> MKSRLKQQIFAISLLACTAISPANALQTHLLREQFQNPSDEAKPWTFWYWMFGAVSKEGITADLEAMKRAGLGGTYLMPIKGIKEGPQYNGKAQQLTPEWWEMVRFSMEEADRLGLKLGMHICDGFALAGGPWMTPKESMQKIVWSDTIVDGGKIKGLHLPQPEAYEGFYEDISLFALPVKEEAADVMPAQITCANIATGNHIDIKKTVNMDDAGVIRSSYPCYIQYEYEQPFTCRNIEIILSGNNYQAHRLKVMASDDGVNYRLVKQLVPARQGWQNTDENSTHAIPATTARYFRFYWTPEGSEPGSEDMDAAKWKPNLKIKELRLHREARLDQWEGKAGLVWRVASSTKKEEIGEQDCYALSQIINLTDPFKNSPSDNFKERTLTATLPKGKWKLLRMGHTATGHTNATAGGGKGLECDKFNPKAVRKQFDNWFAQAFVKTNPDVARRVLKYMHVDSWECGSQNWSDTFAAEFRKRRGYDLMPYLPLLAGIPMESAERSEKILRDVRTTIGELVVDVFYQVLADCAKEYDCQFSAECVAPTMVSDGLLHYQKVDLPMGEFWLNSPTHDKPNDMLDAISGAHIYGKNIIQAEGFTEVRGTW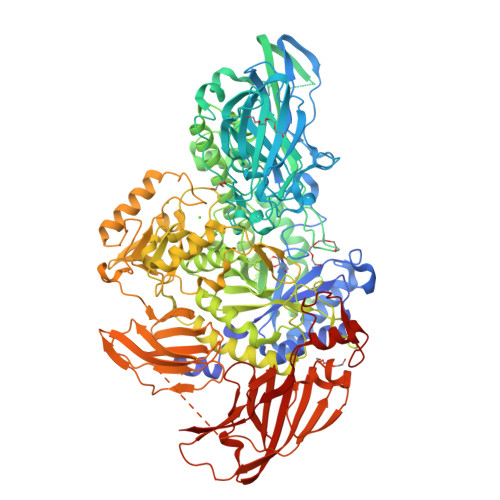NEHPGILKALLDRNYALGINRLFFHVYVHNPWLDRKPGMTLDGIGLFFQRDQTWWNKGAKAFCEYITRCQSLLQYGHPVADIAVFTGEEMPRRSILPERLVPSLPGIFGAERVESERIRLANEGQPLRVRPVGVTHSANMSDPEKWVNPLRGYAYDSFNKDALLRLAKAENGRMTLPGGASYKVLVLPLPRPMNPDPAALSPEVKQKINELKEAGILIPSLPYKEDDFSSYGLERDLIVPENIAWTHRQGEQGDIYFIANQLEETRTFTASMRIDGRKPECWNPVTGEINADIPYEQKSHRTEITLTLAPNESVFIVYPAEEDDKETSEKERKEKKDSVKEASETGLEATEYTVTFTANGKTIQRQELFDWSKEEDEQIRYYSGTAVYKTTFRWKSKVKEDQQVYLNLGKVCDLATVRVNGIDCGTIWTAPYRADITAALKKGVNELEIEVTNTWANALKGADEGKAPFDGIWTNAKYRRAENTLLPAGLLGPLNFDVANKNK> GSDELYRQSLEIISRYLREQATGAKDTKPMGRSGATSRKALETLRRVGDGVQRNHETAFQGMLRKLDIKNEDDVKSLSRVMIHVFSDGVTNWGRIVTLISFGAFVAKHLKTINQESCIEPLAESITDVLVRTKRDWLVKQRGWDG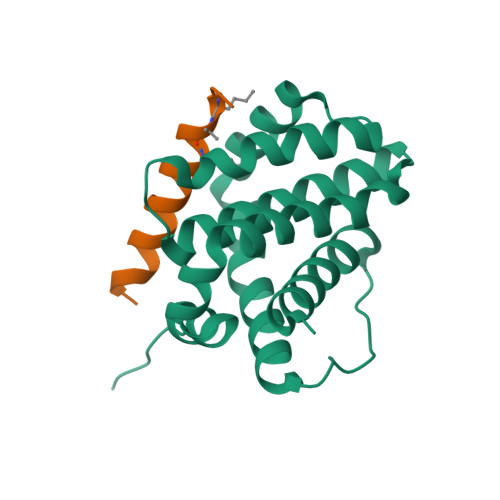FVEFFHVEDLE;> XIWLAQGARRLGDEINAYYARRX>[4x]MSDIKAVAQRALSLMDLTSLTNTETDQEIIDLCRQAKSPAGETAAICIFPRFIPVAKKALKAQQTPHIKIATVTNFPQGNDDLDIALAETRAAVAYGADEVDLVFPYRALIQGNETIGFDMVKVCKQACSGNAKLKVIIETGELKSEELIRKASEIAINAGADFIKTSTGKVAINATPEAAKVMLTVIKNKNTAVGFKPAGGVRNADDAAIYLDLADNILGNEWADANHFRFGASSLLISLLDTLGHKSNTKSSSNYHHHHHH

The 2-deoxy-D-ribose-5-phosphate aldolase (DERA) is an enzyme involved in nucleotide catabolism. The enzyme catalyzes the formation of C-C bonds between an aldehyde as an electrophile and acetaldehyde as a nucleophile in a highly stereoselective manner. The structures display a canonical TIM barrel fold built up of eight β-α repeats in a toroidal arrangement, with an additional N-terminal helix (α0) directly adjacent to the C-terminal helix α8 (vide infra). Furthermore, all DERAs investigated in this study form constitutive dimers.

The X-ray structures of both psychrophilic DERAs were determined with resolutions of 2.1 Å for C. psychrerythraea and 1.8 Å for S. halifaxensis. We note that the relative orientations of protomers as well as the characteristics of the dimer interface for both psychrophilic DERAs closely resemble the situation in the mesophilic (E. coli) enzyme. Comparing the substrate binding pockets of the new structures with DERAEC, no amino acid exchanges or significant conformational differences were found within a radius of 5 Å about the natural substrate (as represented by the covalent intermediate included in PDBID 1JCL12). DERAs from psychrophilic species had a similar thermostability and were around 20 K less stable than DERAEC. In contrast, helices 5 and, particularly, 6 and 7 show markedly reduced strengths of rigid contacts in the psychrophilic enzymes. The relative B-factor distribution of the backbone atoms reveals a tendency towards increased flexibility in helices 0, 6, and 7 of the psychrophilic DERAs, compared to DERAEC. Hence, our X-ray structures provide independent clues in favor of the hypothesis that adaption to low temperatures in psychrophilic DERAs involves a more flexible environment of the substrate binding pocket. While in DERASH and DERAEC the melting point of the oxidized form was still lower than the wt value, the exchange led to a marked increase of 8.4 K in thermostability in the case of DERACP. Further tests for the DERACP-A95Cox variant revealed a much longer half-life at 50 °C (>80 min vs. 1 min for the wt) and 86 ± 8% of the wt activity. Nevertheless, by installing a disulfide bridge in the interface of DERACP as a psychrophilic representative, the melting temperature could be increased.Here we report a detailed structure-function analysis of the kinase ThiM, which phosphorylates THZ in one of the first steps in vitamin B1 biosynthetic pathway. The quaternary structure of SaThiM is a triangular homo-trimer with dimensions of approximately 72 Å on a side and 47 Å thick with three independent active sites, each located within interface regions between two monomers. The following β-sheet strand 7 is antiparallel to strand 6 and following β-sheet strand 8, which is antiparallelly flanked by β-sheet strand 9. This fold of the phosphotransferase ThiM is homologous to that common to the group of ribokinase-like folded kinases. The three active sites, each located within the interface regions of two monomers respectively, are homologous to other known phosphoryl transfer ribokinase-like kinases.

Out of this in silico selected set of molecules, two were chosen as the most promising analogues for further investigations: 2-(1,3,5-Trimethyl-1H-pyrazol-4-yl) ethanol, hereinafter referred to as compound 1 (cpd 1) and 2-(2-Methyl-1H-imidazol-1-yl) ethanol referred to as compound 2 (cpd 2). The structures of these complexes could be refined to 1.87 Å and 1.62 Å resolution with R and Rfree values of 16.86% and 19.90% for the cpd 1 complex and R and Rfree values of 18.24% and 20.28% for the cpd 2 complex. The thiazole moiety was replaced by the non-sulfur containing heterocycles pyrazole and imidazole for cpd 1 and cpd 2, respectively. Moreover, cpd 1 contains two additional methyl groups at position 5 and 6 of the heterocycle (respectively). The overall coordination of the THZ analogue compounds in the active site regions of the ThiM trimer is remarkably comparable to that of the of natural substrate THZ. Both compounds form a H-bond to the amide nitrogen of amino acid M39 and show a similar orientation of their hydroxyethyl groups. The activity of ThiM was analyzed in vitro, as described in the methods section, showing that the specific activities of cpd 1 and cpd 2 are approximately 1.5 times higher compared to THZ, however show only 1/10 of the efficiency (kcat/KM) in comparison to the natural substrate THZ. The two novel compounds applied for co-crystallization in this study lack the thiazolium sulfur, present in the natural thiazolium moiety of thiamin, which is replaced by a carbon atom, supporting slightly higher flexibility in the active site in consequence of the reduced van der Waals radius. Moreover, cpd 1 has two additional methyl groups bound to atoms 1 and 2, which can provide more hydrophobic interactions in binding co-factor dependent enzymes after complexation to the HMP moiety by ThiE thereby enabling the cpd 1-HMP moiety to act as a competitive inhibitor.

>MNYLNNIRIENPLTICYTNDVVKNFTANGLLSIGASPAMSEAPEEAEEFYKVAQALLINIGTLTAQNEQDIIAIAQTANEAGLPIVFDPVAVGASTYRKQFCKLLLKSAKVSVIKGNASEILALIDDTATMKGTDSDANLDAVTIAKKAYAIYKTAIVITGKEDVIVQGDKAIVLANGSPLLARVTGAGCLLGGIIAGFLFRETEPDIEALIEAVSVFNIAAEVAAENENCGGPGTFSPLLLDTLYHLNETTYQQRIRIQEVEENLYQQSGHHHHHH[6x]>AAEAAVTQSPRNKVAVTGEKVTLSC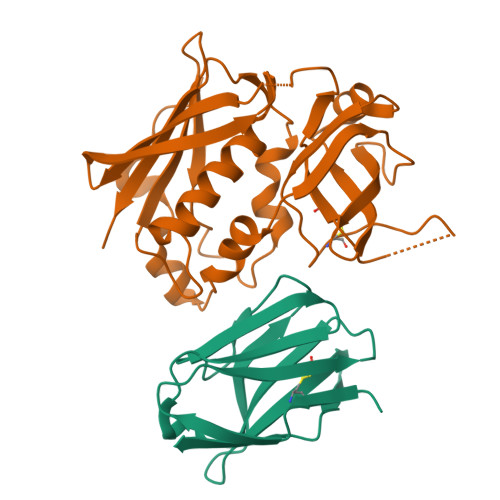QQTNNHNNMYWYRQDTGHGLRLIHYSYGVGNTEKGDIPDGYEASRPSHEQFSLILVSATPSQSSVYFCASGVGGTLYFGAGTRLSVL[8x];>[8x]AQPDPKLDELNKVSDYKSNKGTMGNVMNLYMSPPVEGRGVINSRQFLSHDLIFPIEYKSYNEVKTELENTELANNYKGKKVDIFGVPYFYTCIIPKSEPDINQNFGGCCMYGGLTFNSSENERDKLITVQVTIDNRQSLGFTITTNKNMVTIQELDYKARHWLTKEKKLYEFDGSAFESGYIKFTEKNNTSFWFDLFPKKELVPFVPYKFLNIYGDNKVVDSKSIKMEVFLNTH>[3x]MSKPQPIAAANWKSGSPDSLSGLIDLFNSTSINHDVQCVVASTFVHLAMTKERLSHPKFVIAAQNAGNTDALASLKDFGVNWIVLGHFERRWYYGETNEIVADKVA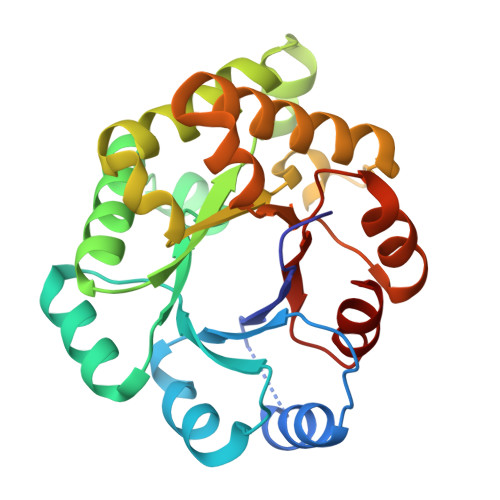AAVASGFMVIACIGETLQERESGRTAVVVLTQIAAIAKKLKKADWAKVVIAYEPVWAIGTGKVVTPQQAQEAHALIRSWVSSKIGADVAGELRILYGGSVNGKNARTLYQQRDVNGFLAGLKPEFVDIIKATQ> MSLKQDLLNDRIILVTGASDGIGREAAMTYARYGATVILLGRNEEKLRQVASHINEETGRQPQWFILDLLTCTSENCQQLAQRIVVNYPRLDGVLHNAGLLGDVCPMSEQNPQVWQDVMQINVNATFMLTQALLPLLLKSDAGSLVFTSSSVGRQGRANWGAYAASKFATEGMMQVLADEYQQRLR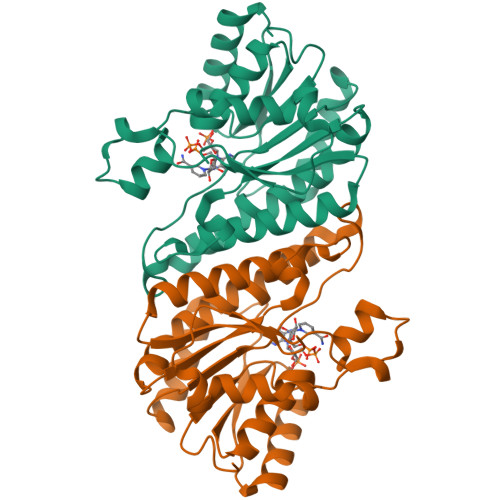VNCINPGGTRTAMRASAFPTEDPQKLKTPADIMPLYLWLMGDDSRRKTGMTFDAQPGRKPGEGHHHHHH> GCNRLN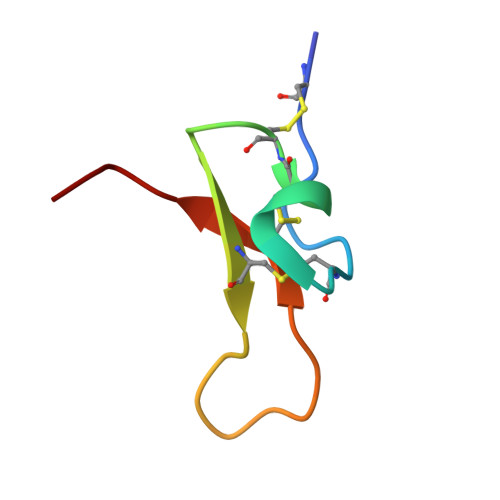KKCNSDADCCANKEKCERPIGWKFMYCRPDVGP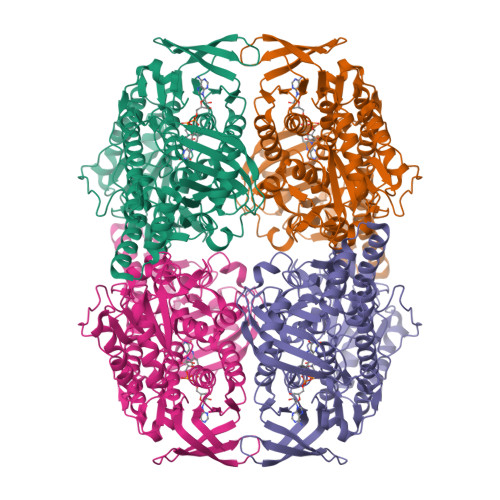>[2x]MHHHHHHSNSAETDVLIVGAGPAGAMSATLLASLGIRSLMINRWRSTSPGPRSHIINQRTMEILRDIGLEESAKSLAVPKEYMGEHVYATSLAGEEFGRIPAWASHPQAHAEHELASPSRYCDLPQLYFEPMVVSEAALRGADVRFLTEYLGHVEDQDGVTARLLDHVSGAEYEVRAKYIIGADGAHSLVAQNAGLPFEGQMGIGDSGSINIEFSADLSSLCEHRKGDMYWMFRAGSGINGVGVAALQMIRPWNKWICVWGYEKSKGTPEITKEEAKKIIHEIIGTDEIPVEVGPISTWTINQQYAVRNTSGRVFCMGDAVHRHTPMGGLGLNTSVQDAYNLAWKLALVLKGTAAPTLLDSYDAERSPVAKQIVERAFKSLSTFPPVFEALSLPPAPTESEMAEALVRLKDASEEGAKRRAALRKAMDATIIGLGGGHGVELNQRYVSRAVFPDGTPDPGFVRDQEFFYQASTRPGAHLPHVWLTENQRRISTLDLCGKGRFTLLTGLSGAAWKHEAEQVSQSLGIELKVCVIGPGQEFVDTYGEYAKISEIGESGALLVRPDMFIAFRAKDASREGLEQLNVAVKSILGRA> ASNLKIVRMDRT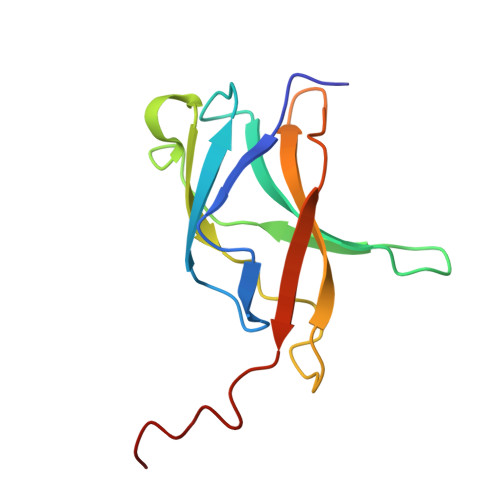AGCVTGGEEIYLLCDKVQKDDIQIRFYEEEENGGVWEGFGDFSPTDVHRQFAIVFKTPKYKDVNITKPASVFVQLRRKSDLETSEPKPFLYYPEIKDKEEVQR> GSHMASSCAVQVKLELGHRAQVRKKPTVEGFTHDWMVFVRGPEHSNIQHFVEKVVFHLHESFPRPKRVCKDPPYKVEESGYAG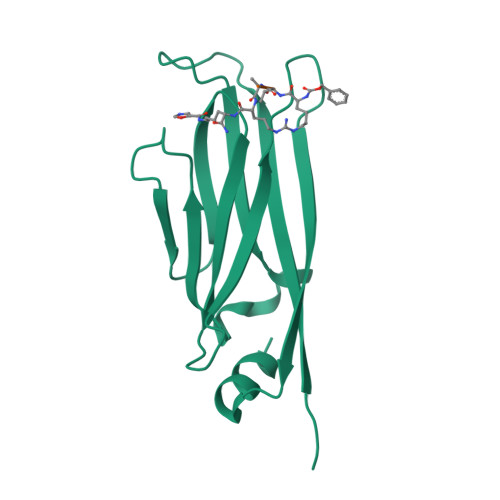FILPIEVYFKNKEEPRKVRFDYDLFLHLEGHPPVNHLRCEKLTFNNPTEDFRRKLLKA>[4x]MGEFEKRAKELIERAKKLNTPAA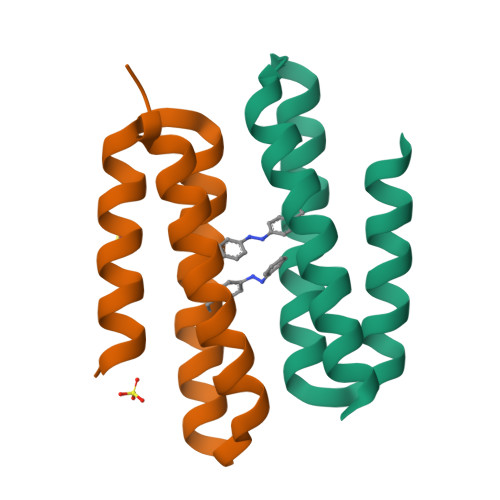KVIEAALKLFIEAYAEAKKKGDALQQKLLEESLKQAEAMLRRLEHHHHHH> VTKPTIAAVGGYAMNNGTGTTLYTKAADTRRSTGSTTKIMTAKVVLAQSNLNLDAKVTIQKAYSDYVVANNASQAHLIVGDKVTVRQLLYGLMLPSGCDAAYALADKYGSGST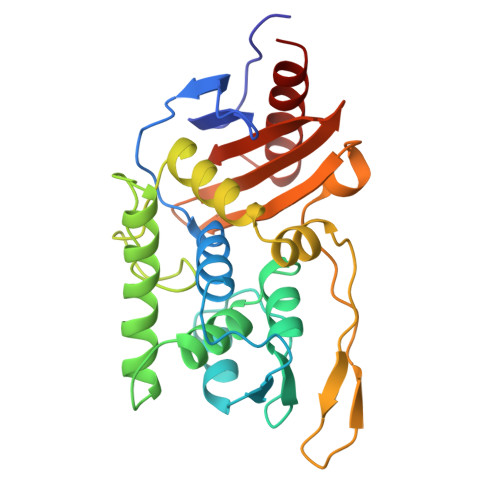RAARVKSFIGKMNTAATNLGLHNTHFDSFDGIGNGANYSTPRDLTKIASSAMKNSTFRTVVKTKAYTAKTVTKTGSIRTMDTWKNTNGLLSSYSGAIGVKTGSGPEAKYCLVFAATRGGKTVIGTVLASTSIPARESDATKIMNYGFAL> MGHHHHHHHHSTGENLYFQGSEVRSYLMEAHSLAGQWSLPNDRGDHTNSEAYDVNSVAIIGGGTMGKAMAICFGLAGIETFLVVRNEQRCKQELEVMYAREKSFKRLNDKRIEKINANLKITSDFHKLSNCDLIVESVIEDMKLKKELFANLENICKSTCIFGTNTSSLDLNEISSVLRDPSNLVGIHFFNPANVIRLVEIIYGSHTSSQAIATAFQACESIKKLPVLVGNCKSFVFNRLLHVYFDQSQKLMYEYGYLPHQIDKIITNFGFLMGPMTVADMNGFDVMEKLKKENGLEPNPIEKEMWRLKRYGRKTNKGFYKYDDKTQRKENDTEMEQIIRRVSQNAKSNIQIINDQDVINFMLYPTVNEGYRCIEEGV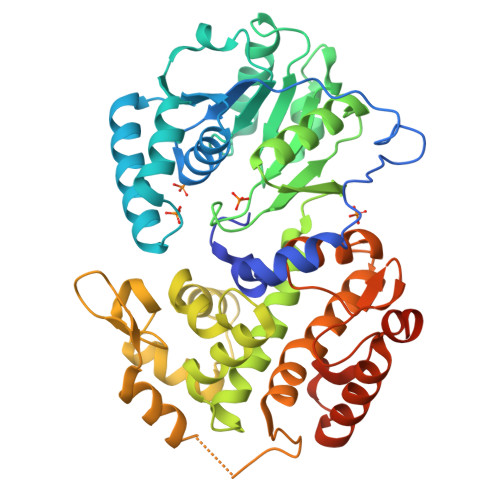ISNESLIDIMFILGFGWPIHSGGPMRFGKTEGLDKIANMLVHWSSLEPKESAYIVADALKTANVSTGSSGSSGGHHHHHHHH> L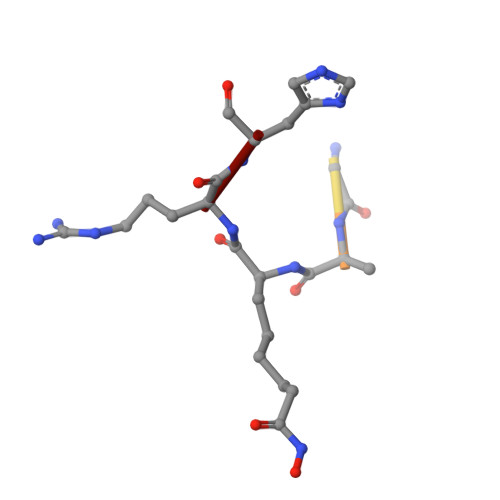GKGGAXRH> GSHMRANELQLRWQEYRELVLLLLQWMRHHTAAFEERRFPSSFEEIEILWSQFLKFKEMELPAKEADKNRSK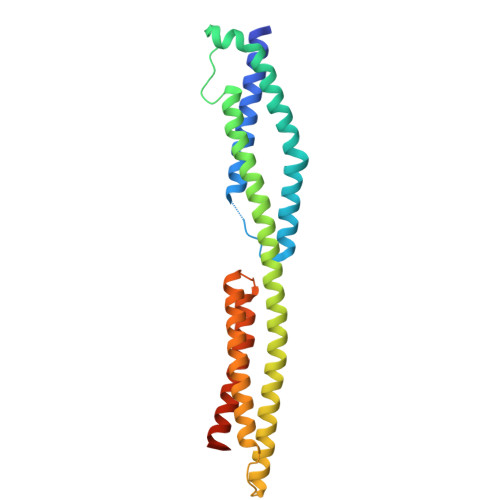GIYQSLEGAVQAGQLKVPPGYHPLDVEKEWGKLHVAILEREKQLRSEFERLECLQRIVTKLQMEAGLCEEQLNQADALLQSDVRLLAAGKVPQRAGEVERDLDKADSMIRLLFNDVQTLKDGRHPQGEQMYRRVYRLHKRLVAIRTEYNLRLKAGVAAPATQV>[3x]MKIATITGVTKSPELQVTKAIGALILSSDVALSALTTEKISIYIERGNGSNVILANKVLLKDFILASTYGTENTQSDADNAMIALCELADEGSIYLADKESIKITLEDLISDKRYDLHGIEEPQQTNNLFFFEQKSVASEEFNKKIDVQGFDLAIMTVDDSVSDLSYQYSNGQVVKYLPFELQTLSRDIDPIQAVLSDGKVVQGLTDRLTLPLVAVVGIEINKSQGSIINFVVRCLKTV

In this study, we report a detailed characterization of ΦCjT23, an icosahedral temperate ssDNA phage with an inner lipid membrane, isolated earlier from a strain of Flavobacterium (previously Cytophaga). The virion structure determined by cryogenic electron microscopy reveals similarities to members of the viral kingdom Bamfordvirae that currently consists solely of dsDNA viruses with a major capsid protein composed of two upright β-sandwiches. The minimalistic structure of ΦCjT23 suggests that this phage serves as a model for the last common ancestor between ssDNA and dsDNA viruses in the Bamfordvirae. Both ΦCjT23 and the related phage FLiP infect Flavobacterium species found in several environments, suggesting that these types of viruses have a global distribution and a shared evolutionary origin.

The basic capsid building block is the pseudo-hexameric MCP trimer. Within the asymmetric unit, type 1 trimers circle the five-fold symmetry axes at the vertices, type 2 trimers reside on both sides of the icosahedral two-fold axis of symmetry, type 3 trimers reside on the icosahedral three-fold axis of symmetry (contributing one MCP per asymmetric unit) and type 4 trimers reside between the rest. We determined the atomic model of ΦCjT23 MCP to compare it with previously determined MCP structures. The improved map quality was sufficient to build atomic models of the trimers de novo. The MCP monomer is composed of two β-sandwiches, V1 (M1–T126) and V2 (N127–V239). The outward-facing EF1-loop is used by trimer 1 to reach under the spike penton domain, and analogously by trimer 2 to reach under trimer 1. The capsid-integral part of the spike, corresponding to the P13 N-terminal penton base domain (residues M1–F91), sits in a slightly raised position relative to the type 1 MCP trimers circling it. Second, pentameric spikes are required to fill the five-fold positions via interactions with peripentonal MCPs.>[2x]MGHHHHHHMGFNSEIKEKYLDTLSEGMVMQMRPIFAKAEITETLYNKDIYDFTSMQILEL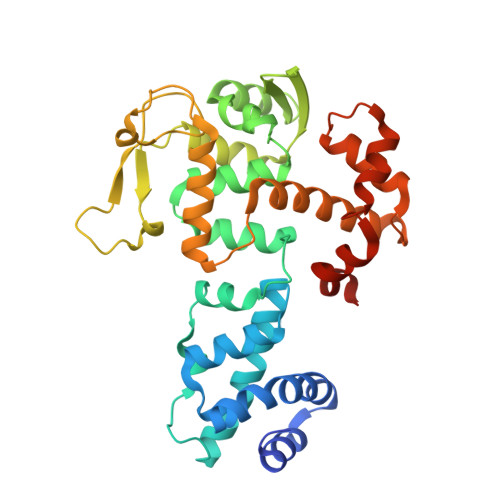IRSFDQTTIGSVRRTLALLSLYIDWAISYKLSKGLTNLARTISEEELYECLGDKKLYITYSELEEMENQLVNYQSKAVLRLLFEGVSGLAHSELLSLTKKQVEDAMLNGNVLTLYDSKHGERKLKVSSECLVIALNAAQETKYKLKNGKAKGQTKEVFLVENDYVVKTKRTSNKGDGQASKFVITNLITDISEFFKINFLTPNTIVRSGHLYRAYQLYKEKGVIDNSVRYQIIDDFNLRVKSKYRAVYSMQDYINEEEVNKYYAEELGLKETTILE> AFAADAGKEVAADVVIGPVLL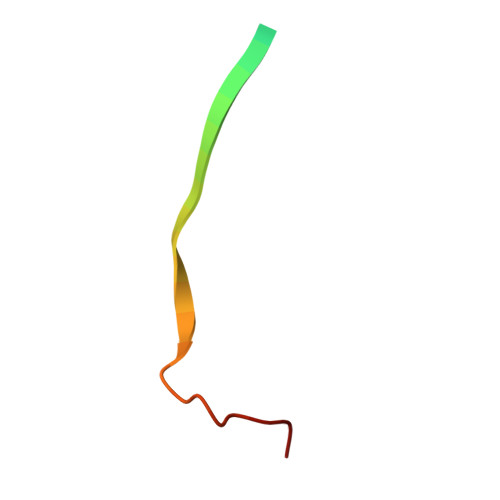SADHHHHHH>TAQIKGLTQAQRNANDGISLAQTAEGALGEISNNLQRIRELAVQASNGTNTQTDRDALQAEVTQLQSEIQRVAEQTSFNGQKLLDGSFNGVQFQIGANAGETIGVSKIMNAQTASLGGSLTRTTSTIDATDLTKYDTAMAAGDLTINGVDVGKIDAASTAQERAAQLTEAINRVSSQTNVGASYDKTTGQVTLTSNAAIAVAGAANDATVAGWANNATTGTATTTTGINSLTVSSFTNAQQTITQIDNALKDINT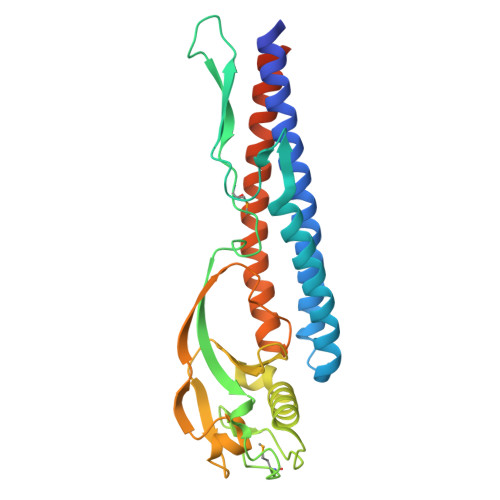ARADLGAVQNRFTSTVANLQSMTENLSSALEHHHHHH[2x]>[4x]GSFVEMVDNLRGKSGQGYYVEMTVGSPPQTLNILVDTGSSNFAVGAAPHPFLHRYYQRQLSS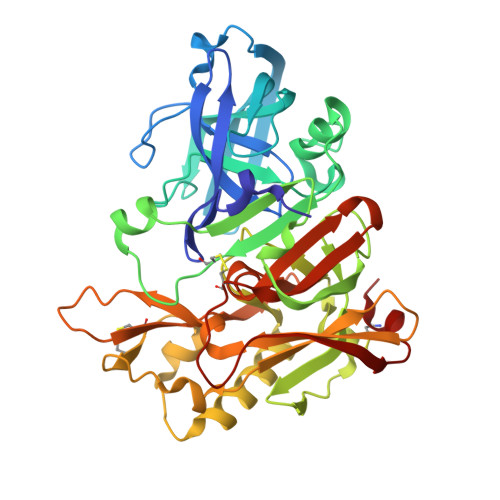TYRDLRKGVYVPYTQGKWEGELGTDLVSIPHGPNVTVRANIAAITESDKFFINGSNWEGILGLAYAEIARPDDSLEPFFDSLVKQTHVPNLFSLQLCGAGFPLNQSEVLASVGGSMIIGGIDHSLYTGSLWYTPIRREWYYEVIIVRVEINGQDLKMDCKEYNYDKSIVDSGTTNLRLPKKVFEAAVKSIKAASSTEKFPDGFWLGEQLVCWQAGTTPWNIFPVISLYLMGEVTNQSFRITILPQQYLRPVEDVATSQDDCYKFAISQSSTGTVMGAVIMEGFYVVFDRARKRIGFAVSACHVHDEFRTAAVEGPFVTLDMEDCGYN>MELKLIPIEKPENLNVILGQAHFIKTVEDLHEALVTAVPGIRFGLAFSEASGKRLVRRSGTDEALVELAVKNLLNLACGHVFLIVLGEGFYPINVLHAVKACPEVVRIYAATANPLKVVVAEEGEQRAILGVMDGFTPLGVEDEAEVAWRKDLLRRLGYKL[6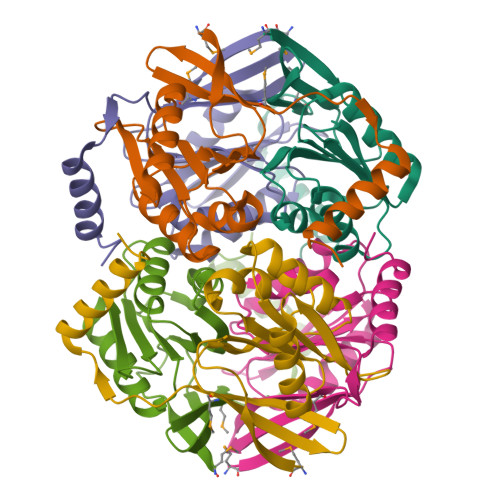x]> LERLVGPQDATHCSPGLSCRLWDSDILCLPGDIVPAPGPVLAPTHLQTELVLRCQKETDCDLCLRVAVHLAVHGHWEEPEDEEKFGGAADSGVEEPRNASLQAQVVLSFQAYPTARCVLLEVQVPAALVQFGQSVGSVVYDCFEAALGSEVRIWSYTQPRYEKELQHTQQLPDCRGLEVWNSIPSCWALPWLNVSADGDNVH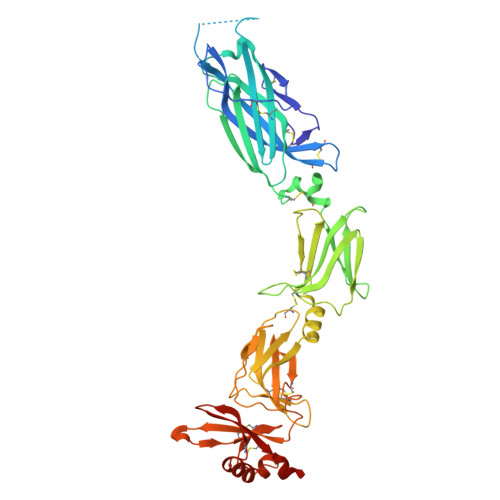LVLQVSEEQHFGLSLYWNQVQGPPKPRWHKQLTGPQIITLQHTDLVPCLCIQVWPLEPDSVRTNICPFREDPRAHQNLWQAARLRLLTLQSWLLDAPCSLPAEAALCWRAPGGDPCQPLVPPLSWEQVTVDKVLEFPLLKGHPNLCVQVQSSEKLQLQECLWADSLGPLKDDVLLLETRGPQDQRSLCALEPSGCTSLPSKASTRAARLGEYLLQDLQSGQCLQLWDDDLGALWACPMDKYIHKREFRH>[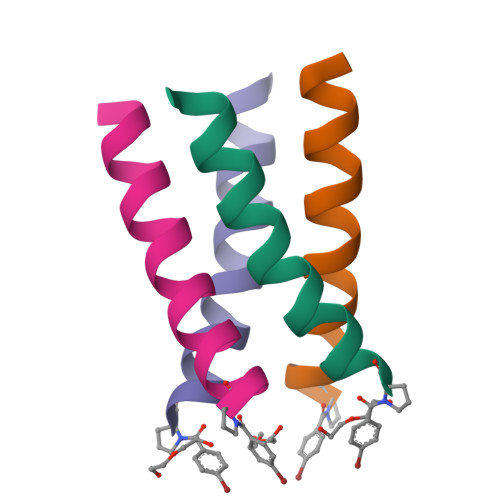4x]PLVVAASIIAILHLILWILDRLX>AQEVLRRTPLYDFHLAHGGKMVAFAGWSLPVQYRDSHTDSHLHTRQHCSLFDVSHMLQTKILGSDRVKLMESLVVGDIAELRPNQGTLSLFTNEAGGILDDLIVTNTSEGHLYVVSNAGCWEKDLALMQDKVRELQNQGRDVGLEVLDNALLALQGPTAAQVLQAGVADDLRKLPFMTSAVMEVFGVSGCRVTRCGYTGEDGVEISVPVAGAVHLATAILKNPEVKLAGLAARDSLRLEAGLCLYGNDIDEHTTPVEGSLSWTLGKRRRAAMDFPGAKVIVPQL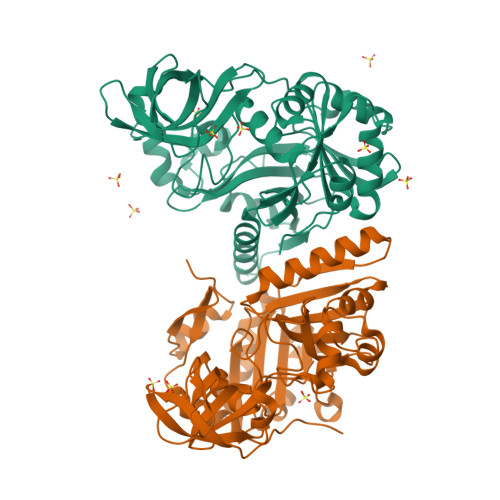KGRVQRRRVGLMCEGAPMRAHSPILNMEGTKIGTVTSGCPSPSLKKNVAMGYVPCEYSRPGTMLLVEVRRKQQMAVVSKMPFVPTNYYTLK[2x]> TQFEERHLKFLQQLGKGNFGSVEMCRYDPLQDNTGEVVAVKKLQHSTEEHLRDFEREIEILKSLQHDNIVKYKGVCYSAGRRNLKLIMEYLPYGSLRDYLQKHKERIDHIKLLQYTSQICKGMEYLGTKRYIHRDLATRNILVENENRVKIGDFGLTKVLPQDKEFFKVKEPGESPIFWYAPESLTESKFSVASDVWSFGVVLYELFTYIEKSKSPPAEFMRMIGNDKQGQSIVTHLIELLKNNGRLPRPDGCPDEIYMIMTE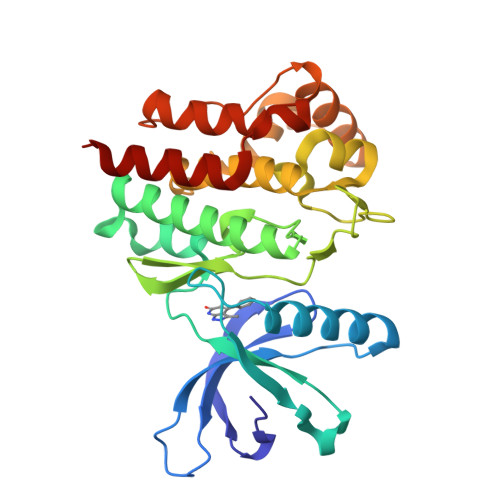CWNNNVNQRPSFRDLALRVDQIRDNM> LNRESVIDAALEL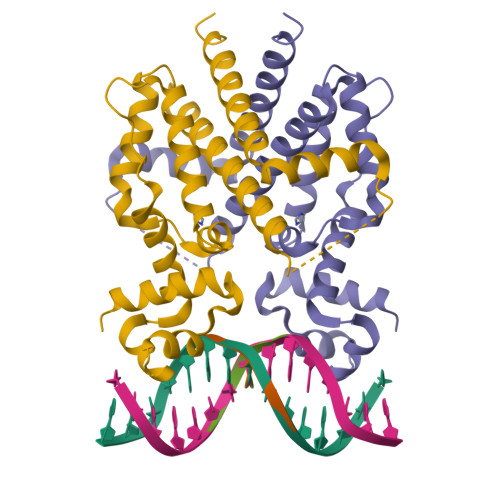LNETGIDGLTTRKLAQKLGIEQPTLYWHVKNKRALLDALAVEILARHHDYSLPAAGESWQSFLRNNAMSFRRALLRYRDGAKVHLGTRPDEKQYDTVETQLRFMTENGFSLRDGLYAISAVSHFTLGAVLEQQEHTAALTDRPAAPDENLPPLLREALQIMDSDDGEQAFLHGLESLIRGFEVQLTALLQ>[2x]MDRSAVDTIRGYCYQVDKTIIEIFSLPQMDDSIDIECIEDVDVYNDGHLTAIQCKYYESTDYNHSVISKPIRLMLSHFKDNKEKGANYYLYGHYKSGQEKLTLPLKVDFFKSNFLTYTEKKIKHEYHIENGLTEEDLQAFLDRLVININAKSFD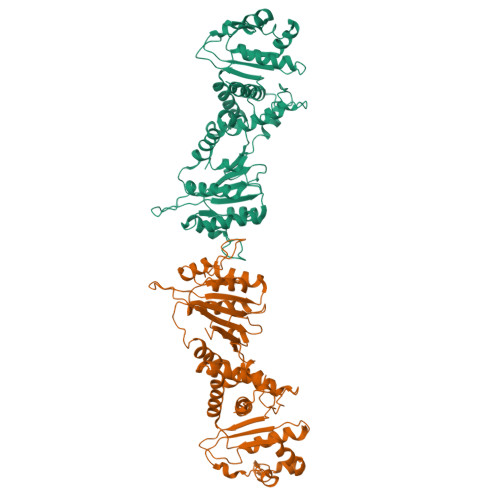DQKKETIQIIKNHFQCEDYEAEHYLYSNAFRKTYDISCNKKDRRIKKSDFVESINKSKVLFNIWFYQYEGRKEYLRKLKESFIRRSVNTSPYARFFILEFQDKTDIKTVKDCIYKIQSNWSNLSKRTDRPYSPFLLFHGTSDANLYELKNQLFNEDLIFTDGYPFKGSVFTPKMLIEGFSNKEIHFQFINDIDDFNETLNSINIRKEVYQFYTENCLDIPSQLPQVNIQVKDFADIKEIV> GQKLSAYVVDWDLPKSIAWDKLDHIVYAFAEPTKDGELSGFTDSQLKSVVQEAHSRGKSISLSVGGWTGSLYFSDLLKSSSSFDNFVSNLVDVVKEYDLDGLNLDWEYPNSPNGVACNSKDENDTANYLKLFKALREKLGSKTILTTAVP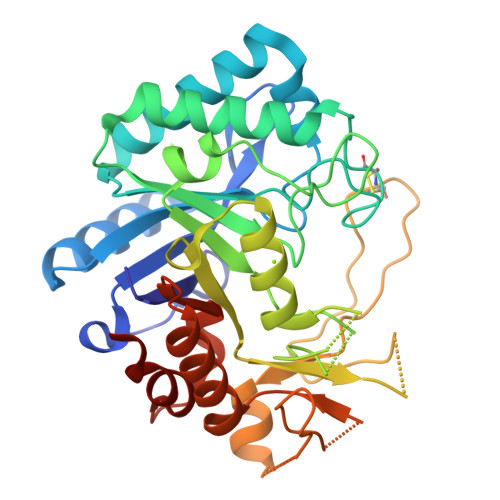TAPFNDENQQPSTKLDDNWASTVDAFYIMAYDVNGIRDKNAGANAPLYYSPKVTGVEPTSGNDAVKAWIAAGIPAEQLVLGVPFYGRVSKTLEPITASTGLYVPISQSSQIKGDSTDEKAADPCPNAVATYSGQYIWRTIAQEGIARNSSGWVTYWDDISKTPYAYSFSGSKVLSFDDAASLQDKVDYAKKQGLGGVMLWSLEMDDDENTLLNALQDIRKLGHHHHHH>[2x]AASEDEFLRYLWRDYLYPKQYAWVLIAAYVAVFVVALVGNTLVCLAVWRNHHMRTVTNYFLVNLSLADVLATAICLPASLLVDITESWLFGHALCKVIPYLQAVSVSVAVLTLSFIALDRWYAICHPLLFKSTARRALGSILGIWAVSLAIMVPQAAVMECSSVLPELAARTRAFSVCDERWADDLAPKIYHSCFFIVTYLAPLGLMAMAYFQIFRKLWGRQIPGTTSAEVKQMRARRKT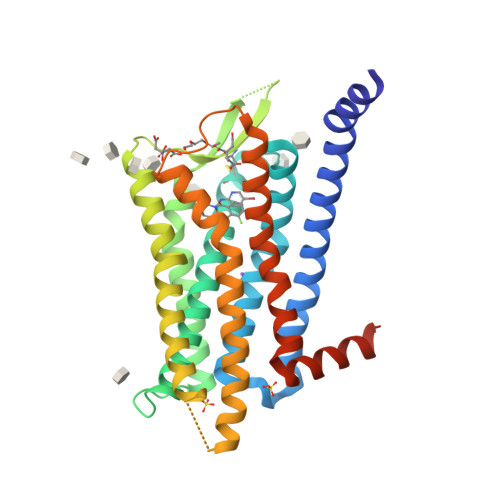AKMLMVVVLVFALCYLPISVLNVLKRVFGMFRQASDREAVYAAFTFSHWLVYANSAANPIIYNFLSGKFREQFKAAFSWWLPGLAAAHHHHHHHHH>[2x]MKLKTTLFGNVYQFKDVKEVLAKANELRSGDVLAGVAAASSQERVAAKQVLSEMTVADIRNNPVIAYEDDCVTRLIQDDVNETAYNQIKNWSISELREYVLSDETSVD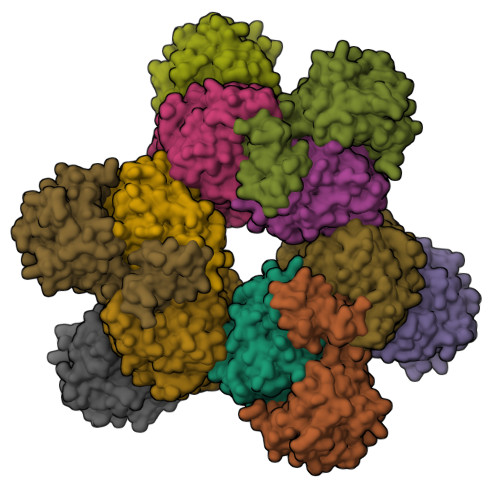DIAFTRKGLTSEVVAAVAKICSNADLIYGAKKMPVIKKANTTIGIPGTFSARLQPNDTRDDVQSIAAQIYEGLSFGVGDAVIGVNPVTDDVENLSRVLDTIYGVIDKFNIPTQGCVLAHVTTQIEAIRRGAPGGLIFQSICGSEKGLKEFGVELAMLDEARAVGAEFNRIAGENCLYFETGQGSALSAGANFGADQVTMEARNYGLARHYDPFIVNTVVGFIGPEYLYNDRQIIRAGLEDHFMGKLSGISMGCDCCYTNHADADQNLNENLMILLATAGCNYIMGMPLGDDIMLNYQTTAFHDTATVRQLLNLRPSPEFERWLESMGIMANGRLTKRAGDPSLFF;>MDQKQIEEIVRSVMASMGQAAPAPSEAKCATTNCAAPVTSESCALDLGSAEAKAWIGVENPHRADVLTELRRSTVARVCTGRAGPRPRTQALLRFLADHSRSKDTVLKEVPEEWVKAQGLLEVRSEISDKNLYLTRPDMGRRLCAEAVEALKAQCVANPDVQVVISDGLSTDAITVNYEEILPPLMAGLKQAGLKVGTPFFVRYGRVKIEDQIGEILGAKVVILLVGERPGLGQSESLSCYAVYSPRMATTVEADRTCISNIHQGGTPPVEAAAVIVDLAKRMLEQKASGINMTR[2x]>EKKSINECDLKGKKVLIRVDFNVPVKNGKITNDYRIRSALPTLKKVLTEGGSCVLMSHLGRPKGIPMAQAGKIRSTGGVPGFQQKATLKPVAKRLSELLLRPVTFAPDCLNAADVVSKMSPGDVVLLENVRFYKEEGSKKAKDREAMAKILASYGDVYISDAFGTAHRDSATMTGIPKILGNGAAGYLMEKEISYFAKVLGNPPRPLVAIVGGAKVSDKIQLLDNMLQRIDYLLIGGAMAYTFLKAQGYSIGKSKCEESKLEFARSLLKKAEDRKVQVILPIDHVCHTEFKAVDSPLITEDQNIPEGHMALDIGPKTIEKYVQTIGKCKSAIWNGPMGVFEMVPYSKGTFAI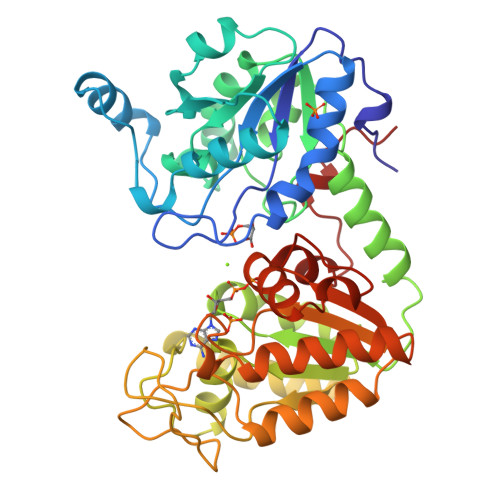AKAMGRGTHEHGLMSIIGGGDSASAAELSGEAKRMSHVSTGGGASLELLEGKTLPGVTVLDDK[4x]(2R,3S,4R)-2-{[4-(3,5-dichlorophenyl)-1H-1,2,3-triazol-1-yl]methyl}pyrrolidine-3,4-diol | C13 H14 Cl2 N4 O2 | 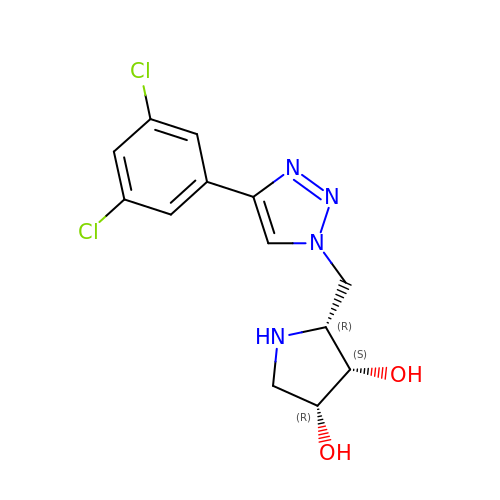QVWPLFTVMWIDFF-UPJWGTAASA-N> ATSTVTGGYAQSDAQGQMNKMGGFNLKYRYEEDNSPLGVIGSFTYTEKSRTASSGDYNKNQYYGITAGPAYRINDWASIYGVVGVGYGKFQTTEYPTYKNDTSDYGFSYGAGLQ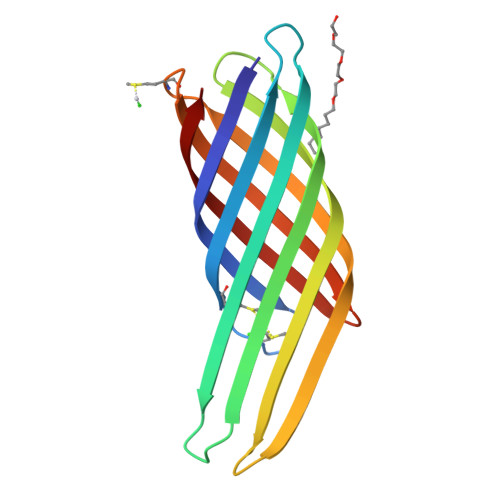FNPMENVALDFSYEQSRIRSVDVGTWIAGVGYRF> MTKEQIQIIKDCVPILQK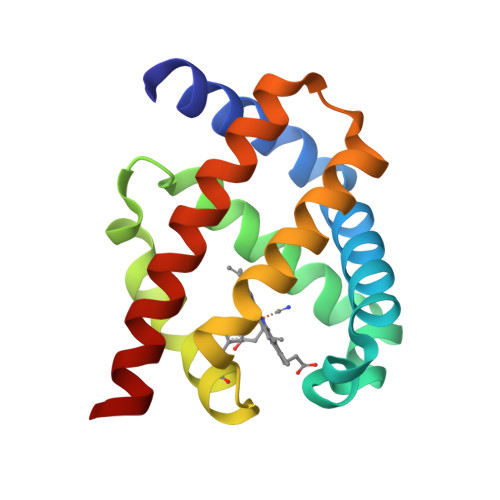NGEDLTNEFYKIMFNDYPEVKPMFNMEKQISGEQPKALAMAILMAAKNIENLENMRSFVDKVAITHVNLGVKEEHYPIVGACLLKAIKNLLNPDEATLKAWEVAYGKIAKFYIDIEKKLYDK The axon initial segment (AIS) has characteristically dense clustering of voltage-gated sodium channels (Nav), cell adhesion molecule Neurofascin 186 (Nfasc), and neuronal scaffold protein Ankyrin-G (AnkG) in neurons, which facilitates generation of an action potential and maintenance of axonal polarity. Among these proteins, Ankyrin-G (AnkG) is considered as the master organizer that directs the recruitment of diverse components to the AIS. In addition, AnkG is also well known to interact with Neurofascin 186 (Nfasc), a cell adhesion molecule that is essential for AIS integrity. Here, we report the high-resolution crystal structure of the AnkG ankyrin repeat (ANK repeat) domain in complex with its binding site in the Nfasc cytoplasmic tail that shows, in conjunction with binding affinity assays with serial truncation variants, the molecular basis of AnkG–Nfasc binding.

In agreement with our understanding of ankyrin structure, the Nfasc ABD peptide extended into the inner groove formed by the ANK repeats. However, in contrast with the antiparallel orientation (N-terminal to C-terminal binding) observed in other ANK repeats–target complex structures reported for ankyrin family proteins (Nav1.2-AnkB, AnkR-AnkB, etc.), the AnkG–Nfasc complex adopted an unexpected parallel binding orientation (i.e., N-terminal to N-terminal binding between Nfasc and ANK repeats). Although we used the Nfasc 1187 to 1214 segment for crystallization, only the Nfasc 1198 to 1214 region could be clearly traced in the electron density map. Unexpectedly, we found that instead of the more easily formed antiparallel intramolecular interaction, the fused Nfasc ABD bound to another AnkG molecule from the neighboring asymmetric unit, forming an intermolecular interaction. Thus, we believed that the parallel binding orientation was not induced by the short covalent linkage but represented the native binding mode. We next examined the specific interactions between residues responsible for their binding and found that the AnkG–Nfasc interface is mainly mediated by hydrophobic and hydrogen bonding interactions. In particular, F1202 from Nfasc inserts into a hydrophobic pocket formed by I277, V282, and C315 from AnkG. Similarly, F1208, another aromatic residue from Nfasc, occupies the hydrophobic groove formed by AnkG residues L343, L376, and V381. Among these, we found that the E1204 sidechain from Nfasc forms hydrogen bonds with T339 and N341 in AnkG, while the main chain of E1204 forms another hydrogen bond with the sidechain of D308 from AnkG. In our solved crystal structure, the corresponding Ser and Tyr residues of Nfasc form 2 hydrogen bonds with H384 from AnkG.

> GPGSEFSDDSLVDYGEGGEGQFNEDGSFIGQYTVGSLVPRGSNDITPLHVASKRGNANMVKLLLDRGAKIDAKTRDGLTPLHCGARSGHEQVVEMLLDRAAPILSKTKNGLSPLHMATQGDHLNCVQLLLQHNVPVDDVTNDYLTALHVAAHCGHYKVAKVLLDKKANPNAKALNGFTPLHIACKKNRIRVMELLLKHGASIQAVTESGLTPIHVAAFMGHVNIVSQLMHHGASPNTTNVRGETALHMAARSGQAEVVRYLVQDGAQV> MSAKDERAREILRGFKLNWMNLRDAETGKILWQGTEDLSVPGVEHEARVPKKILKCKAVSRELNF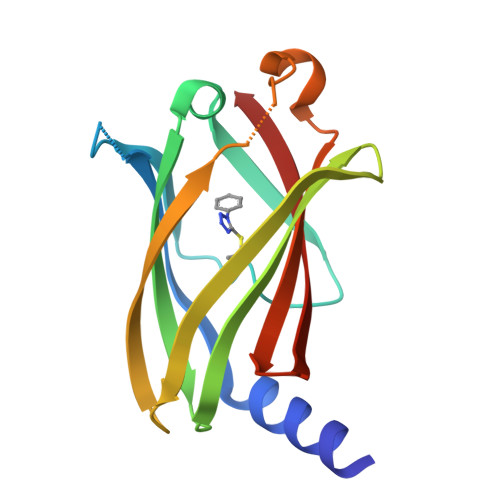SSTEQMEKFRLEQKVYFKGQCLEEWFFEFGFVIPNSTNTWQSLIEAAPESQMMPASVLTGNVIIETKFFDDDLLVSTSRVRLFYV> MIVILDNGGQYVHRIHRSLKYIGVSSKIVPNTTPLEEIESNKEVKGIILSGGPDIEKAKNCIDIALNAKLPILGICLGHQLIALAYGGEVGRAEAEEYALTKVYVDKENGLFKNVPREFNAWASHKDEVKKVPEGFEIL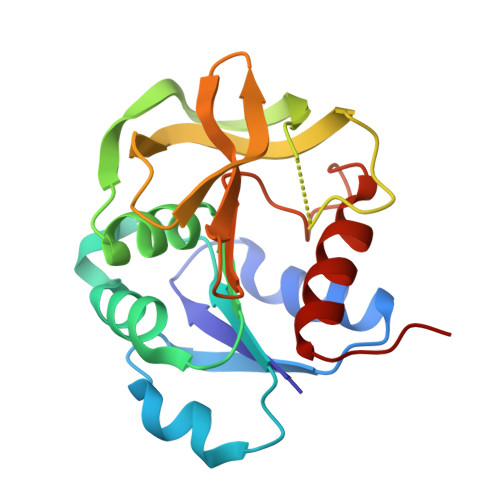AHSDICQVEAMKHKTKPIYGVQFHPEVAHTEYGNEILKNFCKVCGYKFE> MHHHHHHHAVRASEISRVYEAYPEKKATLYFLVLGFLALIVGSLFGPFQALNYGNVDAYPLLKRLLPFVQSYYQGLTLHGVLNAIVFTQLFAQAIMVYLPARELNMRPNMGLMWLSWWMAFIGLVVFALPLLANEATVLYTFYPPLKGHWAFYLGASVFVLSTWVSIYIVLDLWRRWKAANPGKVTPLVTYMAVVFWLMWFLASLGLVLEAVLFLLPWSFGLVEGVDPLVARTLFWWTGHPINYFWLLPAYAIIYTILPKQAGGKLVSDPMARLAFLLFLLLSTPVGFHHQFADPGIDPTWKMIHSVLTLFVAVPSLMTAFTVAASLEFAGRLRGGRGLFGWIRAL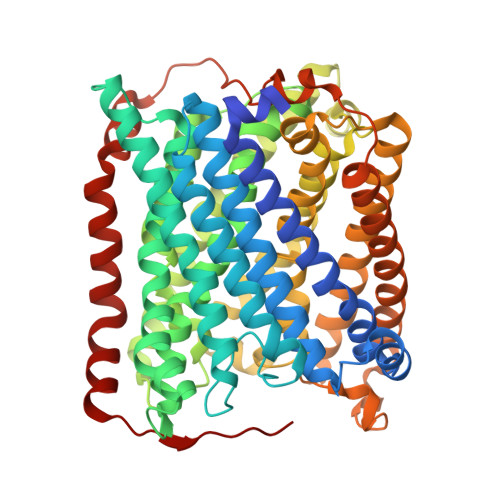PWDNPAFVAPVLGLLGFIPGGAGGIVNASFTLDYVVHNTAWVPGHFHLQVASLVTLTAMGSLYWLLPNLTGKPISDAQRRLGLAVVWLWFLGMMIMAVGLHWAGLLNVPRRAYIAQVPDAYPHAAVPMVFNVLAGIVLLVALLLFIYGLFSVLLSRERKPELAEAPLPFAEVISGPEDRRLVLAMDRIGFWFAVAAILVVLAYGPTLVQLFGHLNPVPGWRLW>MSSKSDDFGSIVASGVTGSGDGNGNGNDWVEKAKDVLQTSVDAVTETAKKTKDVSDEMIPHVQQFLDSNPYLKDVIVPVSLTMTGTLFAWVVMPRILRRFHTYAMQSSAKLLPVGFSNEDVPYEKSFWGALEDPARYLVTFIAFAQIAAMVAPTTIAAQYFSPTVKGAVILSLVWFLYRWKTNVITRMLSAKSFGGLDREKVLTLDKVSSVGLFAIGLMASAEACGVAVQSILTVGGVGGVVTAFAARDILGNVLSGLSMQFSRPFSMGDTIKAGSVEGQVIEMGLTTTSLLNAEKFPVLVPNSLFSSQVIVNKSRAQWRAIASKIPLQIDDLDMIPQISNEIKEMLRSNTKVFLGKEAPHCYLSRVEKSFAELTIGCNLIRMGKEELYNTQQEVLLEAVKIIKKHGVSLGTTWDNSTLSNSLEVLFQ[7x]

MSL1, predicted to contain five transmembrane helices and localized to the inner membranes of mitochondria, is involved in the regulation of membrane potential and maintenance of redox homeostasis under abiotic stress. When heterologously expressed in giant E. coli spheroplasts, MSL1 displays stretch-activated gating in excised patches and channel properties similar to those of E. coli MscS (EcMscS), which demonstrates that MSL1 forms a functional mechanosensitive channel. The overall architecture and domain organization of the heptameric AtMSL1 channel resemble those of the EcMscS channel. Akin to TM3 in EcMscS, the innermost helix TM5 is kinked such that TM5a lines the pore and TM5b runs tangentially to the central pore axis and connects to the middle and C-terminal domains, which are located in the mitochondrial matrix.

Electrophysiological analyses of EcMscS, AtMSL1, and AtMSL1 A320V expressed in giant E. coli spheroplasts indicated that AtMSL1 A320V exhibits much longer open dwell times (that is, the amount of time spent in the open or partially open states) upon tension release than AtMSL1 when gating is triggered by a brief application of negative pressure. We determined the cryo-EM structure of the AtMSL1 A320V mutant in detergents to an overall resolution of ~3.0 Å. The bowl-shaped transmembrane region observed in the wild-type channel flattens, which is accompanied by considerable in-plane expansion. In the structure of A320V in detergents, the diameter of the transmembrane domain is increased from 90 to 105 Å while the height of the channel is reduced from 116 to 92 Å, compared with those in the wild-type structure. These drastic global conformational changes in the transmembrane domain result in substantial opening of the central pore, which increases in diameter from ~8 Å in the wild type to ~20 Å in A320V. The pore-lining helix TM5a becomes more tilted within the membrane and joins TM5b without an apparent kink. Concomitantly, the outward movement of the straightened TM5 helix results in wide opening of the hydrophobic gate, which renders the conduction path less hydrophobic at this region.>MALVCEGKRSASCPCFFLLTAKFYWILTMMRTHSQEYAHSIRVDGDIILGGLFPVHAKGERGVPCGELKKEKGIHRLEAMLYAIDQINKDPDLLSNITLGVRILDTCSRDTYALEQSLTFVQALIEKDASDVKCANGDPPIFTKPDKISGVIGAAASSVSIMVANILRLFKIPQISYASTAPELSDNTRYDFFSRVVPPDSYQAQAMVDIVTALGWNYVSTLASEGNYGESGVEAFTQISREIGGVSIAQSQKIPREPRPGEFEKIIKRLLETPNARAVIMFANEDDIRRILEAAKKLNQSGHFLWIGSDSWGSKIAPVYQQEEIAEGAVTILPKRASIDGFDRYFRSRTLANNRRNVWFAEFWEENFGCKLGSHGKRNSHIKKCTGLERIARDSSYEQEGKVQFVIDAVYSMAYALHNMHKDLCPGYIGLCPRMSTIDGKELLGYIRAVNFNGSAGTPVTFNENGDAPGRYDIFQYQITNKSTEYKVI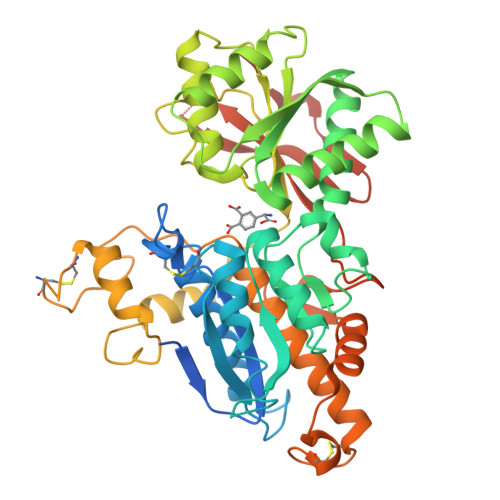GHWTNQLHLKVEDMQWAHRENLYFQGEGHHHHHH[2x]>MGKEALLNLYRIEYRPKDTTFTVFKPTHEIQKEKLNKVRWRVFLQTGLPTFRREDEFWCAGKVEKDTLYLTLSNGEIVELKRVGEEE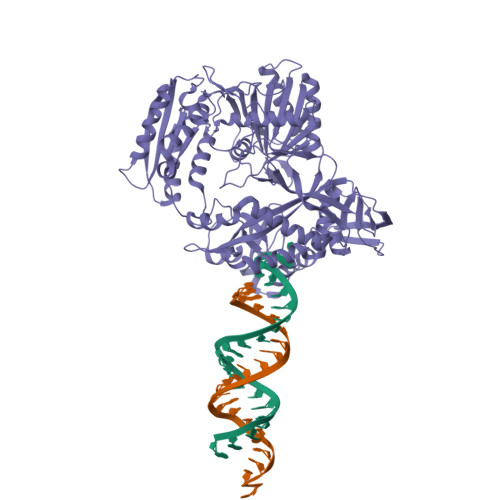FRGFQNERECQELFRDFLTKTKVKDKFISDFYKKFRDKITVQGKNRKIALIPEVNEKVLKSEEGYFLLHLDLKFRIQPFETLQTLLERNDFNPKRIRVKPIGIDFVGRVQDVFKAKEKGEEFFRLCMERSTHKSSKKAWEELLKNRELREKAFLVVLEKGYTYPATILKPVLTYENLEDEERNEVADIVRMEPGKRLNLIRYILRRYVKALRDYGWYISPEEERAKGKLNFKDTVLDAKGKNTKVITNLRKFLELCRPFVKKDVLSVEIISVSVYKKLEWRKEEFLKELINFLKNKGIKLKIKGKSLILAQTREEAKEKLIPVINKIKDVDLVIVFLEEYPKVDPYKSFLLYDFVKRELLKKMIPSQVILNRTLKNENLKFVLLNVAEQVLAKTGNIPYKLKEIEGKVDAFVGIDISRITRDGKTVNAVAFTKIFNSKGELVRYYLTSYPAFGEKLTEKAIGDVFSLLEKLGFKKGSKIVVHRDGRLYRDEVAAFKKYGELYGYSLELLEIIKRNNPRFFSNEKFIKGYFYKLSEDSVILATYNQVYEGTHQPIKVRKVYGELPVEVLCSQILSLTLMNYSSFQPIKLPATVHYSDKITKLMLRGIEPIKKEGDIMYWL[2x]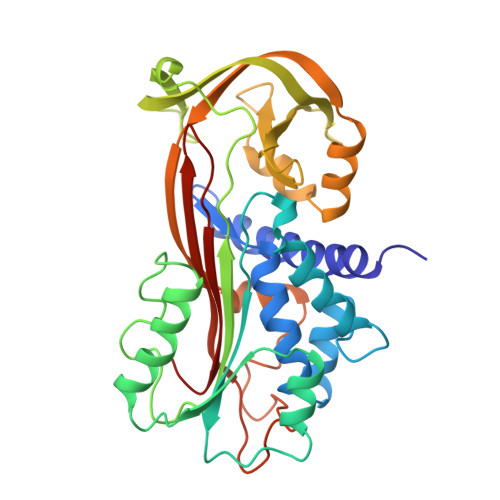> VHHPPSYVAHLASDFGVRVFQQVAQASKDRNVVFSPYGVASVLAMLQLTTGGETQQQIQAAMGFKIDDKGMAPALRHLYKELMGPWNKDEISTTDAIFVQRDLKLVQGFMPHFFRLFRSTVKQVDFSEVERARFIINDWVKTHTKGMISNLLGKGAVDQLTRLVLVNALYFNGQWKTPFPDSSTHRRLFHKSDGSTVSVPMMAQTNKFNYTEFTTPDGHYYDILELPYHGDTLSMFIAAPYEKEVPLSALTNILSAQLISHWKGNMTRLPRLLVLPKFSLETEVDLRKPLENLGMTDMFRQFQADFTSLSDQEPLHVAQALQKVKIEVNESGTVPSSSTAVIVSAR>MSRIVNVKLSLKRYEYEKPFHITGSVSSESRNVEVEIVLESGVKGYGEASPSFRVNGERVEALLAIENAVREMITGIDVRNYARIFEITDRLFGFPSLKAAVQFATLDALSQELGTQVCYLLGGKRDEIETDKTVGIDTVENRVKEAKKIFEEGFRVIKIKVGENLKEDIEAVEEIAKVTRGAKYIVDANMGYTQKEAVEFARAVYQKGIDIAVYEQPVRREDIEGLKFVRFHSPFPVAADESARTKFDVMRLVKEEA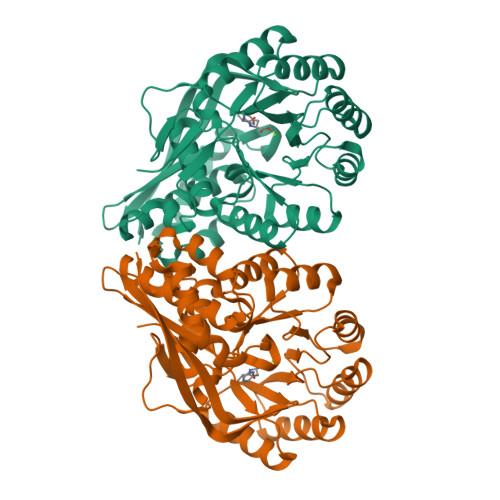VDYVNIKLMKSGISDALAIVEIAESSGLKLMIGCMGESSLGINQSVHFALGTGAFEFHDLDSHLMLKEEVFRGKFIQDGPRMRVKDQ[4x]>[2x]MAGDTTITVVGNLTADPELRFTPSGAAVANFTVASTPRMFDRQSGE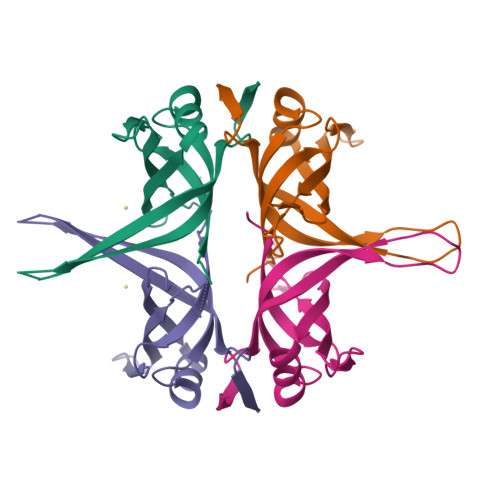WKDGEALFLRCNIWREAAENVAESLTRGSRVIVTGRLKQRSFETREGEKRTVVEVEVDEIGPSLRYATAKVNKASRSGGGGGGFGSGGGGSRQSEPKDDPWGSAPASGSFSGADDEPPF>[2x]MYYLGKELQKRSEELSRGFYELVYPPVDMYEEGGYLVVVADLAGFNKEKIKARVSGQNELIIEAEREITEPGVKYLTQRPKYVRKVIRLPYNVAKDAEISGKYENGVLTIR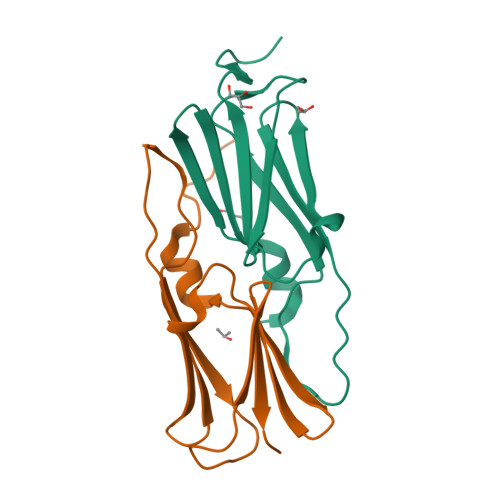IPIAGTSVFKFE>MRVLALSAVFLVASIIGMPAVAKEWQENKSWNAHFTEHKSQGVVVLWNENKQQGFTNNLKRANQAFLPASTFKIPNSLIALDLGVVKDEHQVFKWDGQTRDIATWNRDHNLITAMKYSVVPVYQEFARQIGEARMSKMLHAFDYGNEDISGNVDSFWLDGGIRISATEQISFLRKLYHNKLHVSERSQRIVKQA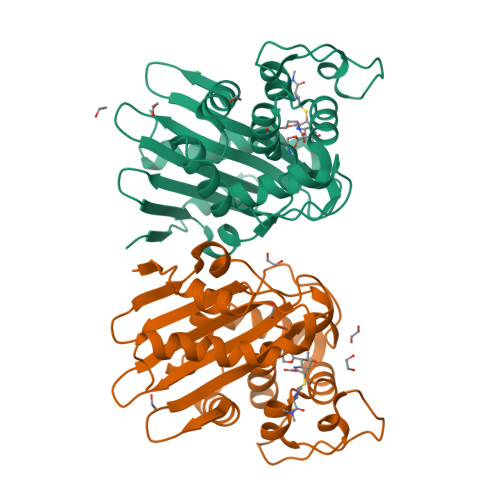MLTEANGDYIIRAKTGYSTRIEPKIGWWVGWVELDDNVWFFAMNMDMPTSDGLGLRQAITKEVLKQEKIIP[4x]>MNLEKFVDELPIPEVAEPVKKNPRQTYYEIAMEEVFLKVHRDLPPTKLWTYNGSLPGPTIHANRNEKVKVKWMNKLPLKHFLPVDHTIHEGHHDEPEVKTVVHLHGGVTPASSDGYPEAWFSRDFEATGPFFEREVYEYPNHQQACTLWYHDHAMALTRLNVYAGLAGFYLISDAFEKSLELPKDEYDIPLMIMDRTFQEDGALFYPSRPNNTPEDSDLPDPSIVPFFCGETILVNGKVWPYLEVEPRKYRFRILNASNTRTYELHLDNDATILQIGSDGGFLPRPVHHQSFTIAPAERFDVI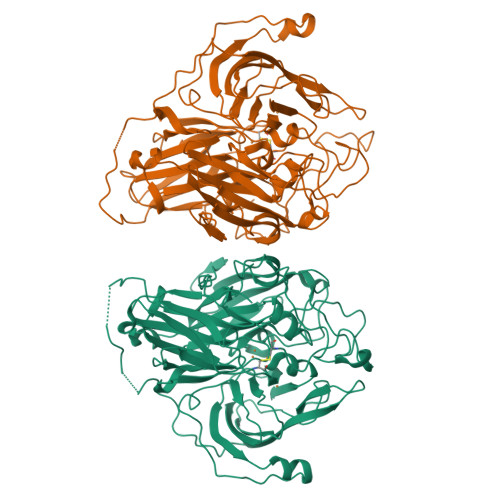IDFSAYENKTITLKNKAGCGQEVNPETDANIMQFKVTRPLKGRAPKTLRPIFKPLPPLRPSRADQERTLTLTGTQDKYGRPILLLDNHFWNDPVTENPRLGSVEVWSIVNPTRGTHPIHLHLVQFRVIDRRPFDTEVYQSTGDIVYTGPNEAPPLHEQGYKDTIQAHAGEVIRIIARFVPYSGRYVWHCHILEHEDYDMMRPMDIIHHHHHH[2x]> GSHMDKLPIEETLEDSPQTRSLLGVFEEDATAISNYMNQLYQAMHRIYDAQNELSAATHLTSKLLKEYEKQRFPLGGDDEVMSSTLQQFSKVIDELSSCHAVLSTQLADAMMFPITQFKERDLKEILTLKEVFQIASNDHDAAINRYSRLSKKRENDKVKYEVTEDVYTSRKKQHQTMMHYFCA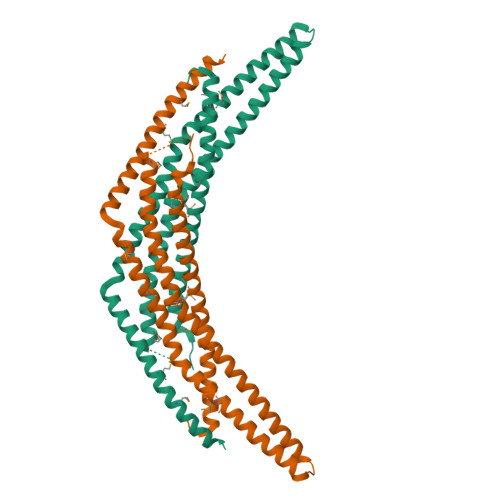LNTLQYKKKIALLEPLLGYMQAQISFFKMGSENLNEQLEEFLANIGTSVQNVRREMDSDIETMQQTIEDLEVASDPLYVPD> MGSSHHHHHHSQGSMERKISRIHLVSEPSITHFLQVSWEKTLESGFVITLTDGHSAWTGTVSESEISQEADDMAMEKGKYVGEL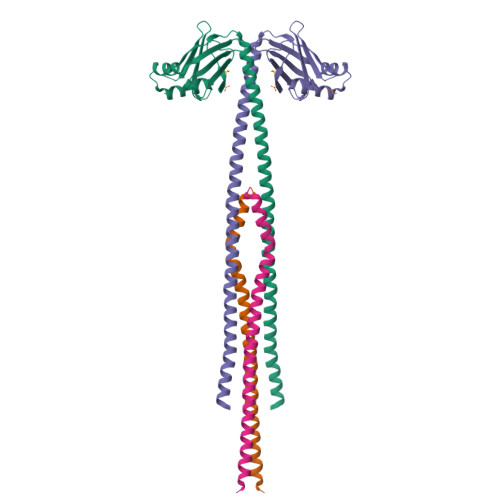RKALLSGAGPADVYTFNFSKESCYFFFEKNLKDVSFRLGSFNLEKVENPAEVIRELICYCLDTIAENQAKNEHLQKENERLLRDWNDVQGRFEKCVSAKEALETDLYKRFILVLNEKKTKIRSLHNKLLNAAQEREKDIKQEG;> MARSMEQQEDSLEKVIKDTESLFKTREKEYQETIDQIELELATAKNDMNRHLHEYMEMCSMKRGLDVQMETCRRLITQSGDR PHOSPHORIC ACID MONO-[5-({[5-CARBAMOYL-3-(5-PHOSPHONOOXY-5-DEOXY-RIBOFURANOSYL)- 3H-IMIDAZOL-4-YLAMINO]-METHYL}-AMINO)-2,3,4-TRIHYDROXY-PENTYL] ESTER | 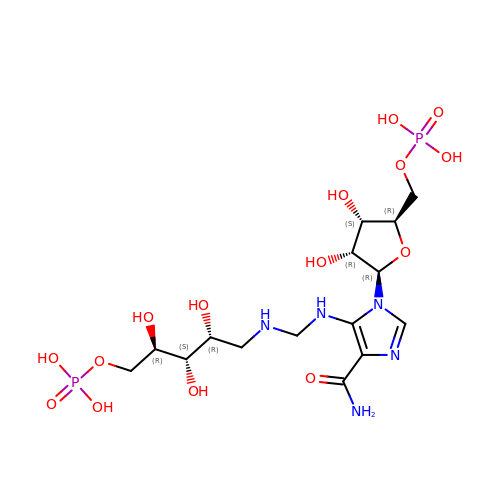C15 H29 N5 O15 P2 | HDCXLRQQJHBDSI-DYHIIFNWSA-N>GMSAKAAEGYEQIEVDVV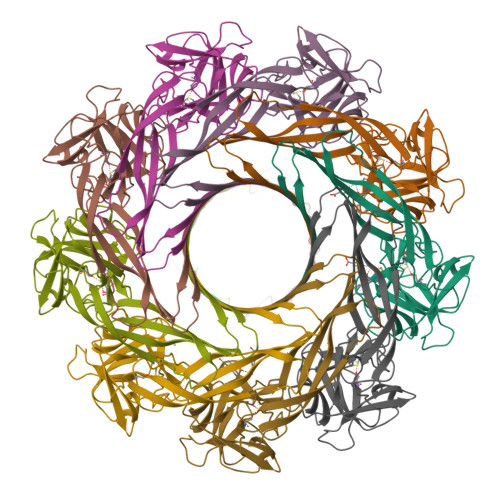AVWKEGYVYENRGSTSVDQKITITKGMKNVNSETRTVTATHSIGSTISTGDAFEIGSVEVSYSHSHQKSQVSMTQTEVYSSKVIEHTITIPPTSKFTRWQLNADVGGAGIEYMYLIDEVTPIGGTQSIPQVITSRAKIIVGRQIILGKTEIRIKHAERKEYMTVVSRKSWPAATLGHSKLFKFVLYEDWGGFRIKTLNTMYSGYEYAYSSDQGGIYFDQGTDNPKQRWAINKSLPLRHGDVVTFMNKYFTRSGLCYDDGPATNVYCLDKREDKWILEVVG[18x]The innate immune protein human surfactant protein D (hSP-D) is a collagenous C-type lectin prototypically associated with the lung surfactant but now identified throughout the human body. SP-D recognises a wide range of pathogens, through their surface carbohydrate arrays, leading to rapid deactivation and clearance through activation of phagocytic cells. Numerous studies of the binding of simple sugars to both hSP-D and rfhSP-D, a recombinant homotrimeric native fragment comprised of the neck region plus three carbohydrate recognition domains (CRDs) which exhibits significant biological and therapeutic activity in vivo and in vitro have been carried out both in solution and through 3-dimensional structural studies. Here we show that hSP-D recognition of Salmonella enterica sv Minnesota rough strains R5 and R7 (rough mutant chemotypes Rc and Rd1) LPS occurs preferentially through the inner core Hep-Kdo, with hSP-D having the flexibility and versatility to target the terminal glucose of R5 when the preferred epitope is not accessible for binding.

The trimeric rfhSP-D structures comprising three carbohydrate recognition domains (CRDs) and the α-helical coiled-coil neck region have been refined to 1.65 Å and 1.75 Å resolution for the R5-bound and R7-bound structures respectively. In all but one of the CRDs the structures reveal oligosaccharide ligand in the Ca1 binding pocket. No ligand is present in subunit A of the R7-bound structure while the mode of oligosaccharide recognition in subunit A of the R5-bound structure differs from the Hep-Kdo binding seen in subunits B and C of both structures. The bound oligosaccharide is clearly defined in the electron density of both structures; Kdo-HepI-HepII for the R7 and Kdo-HepI-HepII-Glc1 for R5. The Kdo electron density clearly shows the 2-oxobutanoic acid sidechain off C4 in a beta conformation with respect to the glycosidic bond in both structures. In subunits B and C, in both structures, recognition of the oligosaccharide by rfhSP-D is primarily via protein and Ca1 coordination of the 6'OH and 7'OH of the dihydroxyethyl side chain of HepI. For both ligands where HepI is coordinated to Ca1 (subunits B and C, both structures) the Kdo (anhydro) interacts with both binding site flanking residues, forming hydrogen bonds with Asp325 through Kdo O6 (2.56–2.80 Å) and with Arg343 through the extended 2-oxobutanoic acid sidechain of the anhydro Kdo. In all subunits where the carbohydrate binding site is openly accessible in the crystal (subunits B and C, both structures), HepI is coordinated to calcium Ca1 as reported for the H. influenzae Eagan 4A –rfhSP-D structure with KdoI extending between the two binding-site flanking residues, Asp325 and Arg343, both of which interact directly with the bound HepI-Kdo (anhydro) unit.

>[3x]GSPGLKGDKGIPGDKGAKGESGLPDVASLRQQVEALQGQVQHLQAAFSQYKKVELFPNGQSVGEKIFKTAGFVKPFTEAQLLCTQAGGQLASPRSAAENAALQQLVVAKNEAAFLSMTDSKTEGKFTYPTGESLVYSNWAPGEPNDDGGSEDCVEIFTNGKWNDRACGEKRLVVCEF>GSSHHHHHHSSGENLYFQGHMTCPFADPAALYSRQDTTSGQSPLAAYEVDDSTGYLTSDVGGPIQDQTSLKAGIRGPTLLEDFMFRQKIQHFDHERVPERAVHARGAGAHGTFTSYADWSNITAASFLNATGKQTPVFVRFSTTAGSRGSADTARDVHGFATRFYTDEGNFDIVGNNIPVFFIQDAIQFPDLIHSVKPRPDNEIPQAATAHDSAWDFFSQQPSTMHTLFWAMSGHGIPRSYRHMDGFGVHTFRFVKDDGSSKLIKWHFKSRQGKASLVWEEAQVLSGKNADFHRQDLWDAIESGNGPEWDVCVQIVDESQAQAFGFDLLDPTKIIPEEYAPLTKLGLLKLDRNPTNYFAETEQVMFQPGHIVRGIDFTEDPLLQGRLFSYLDTQLNRNGGPNFEQLPINMPRVPIHNNNRDGAGQMFIHRNKYPYTPNTLNSGYPRQANQNAGRGFFTAPGRTASGALVREVSPTFNDHWSQPRLFFNSLTPVEQQFLVNAMRFEISLVKSEEVKKNVLTQLNRVSHDVAVRVAAAIGLGAPDADDTYYHNNKTAGVSIVGSGPLPTIKTLRVGILATTSESSALDQAAQLRTRLEKDGLVVTVVAETLREGVDQTYSTADATGFDGVVVVDGAAALFASTASSPL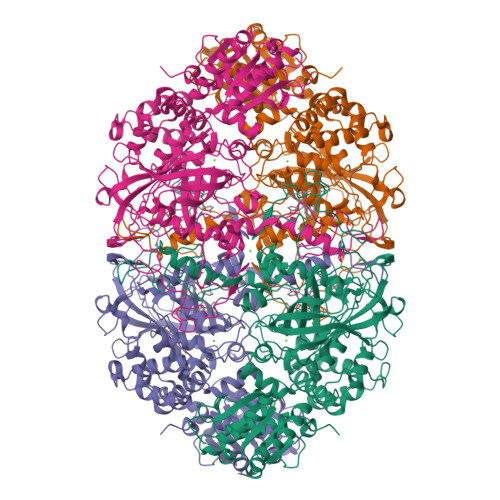FPTGRPLQIFVDAYRWGKPVGVCGGKSSEVLDAADVPEDGDGVYSEESVDMFVEEFEKGLATFRFTDRFALDS[4x]> ASQPPQVTVDKLKRLENDFGGRIGVYAIDTGSNKTFGYRANERFPLCSSFKGFLAAAVLSKSQQQEGLLNQRIRYDNRVMEPHSPVTEKQITTGMTVAELSAATLQYSDNGAA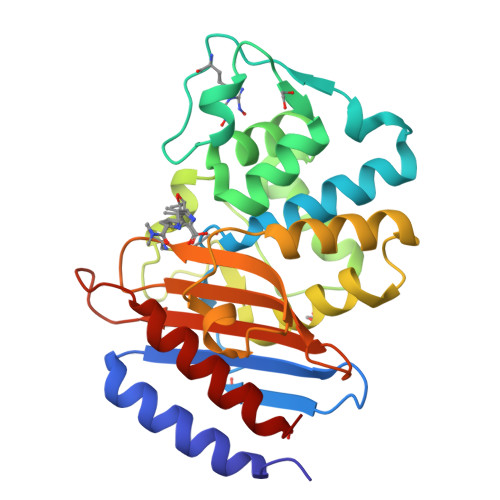NLLLEKLIGGPEGMTSFMRSIGDNVFRLDRWALELNSAIPGDDRDTSTPKAVAESMQKLAFGNVLGLTERHQLMDWFKGNTTGGARIRASVPANWVVGDKTGTCGVYGTANDYAVIWPVAHAPIVLAVYTSKPDRNSKHSDAVIADASRIVLESFNI> MEQLTKCEVFQKLKDLKD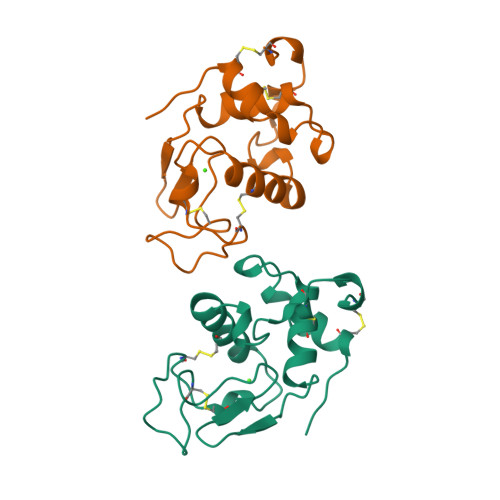YGGVSLPEWVCTAFHTSGYDTQAIVQNNDSTEYGLFQINNKIWCKDDQNPHSRNICNISCDKFLDDDLTDDIVCAKKILDKVGINYWLAHKALCSEKLDQWLCEKL>[3x]METLFSGIQPSGIPTIGNYIGALKQFVDVQNDYDCYFCIVDQHAITMPQDRLKLRKQTRQLAAIYLASGIDPDKATLFIQSEVPAHVQAGWMLTTIASVGELERMTQYKDKAQKAVEGIPAGLLTYPPLMAADIVLYNTNIVPVGDDQKQHIELTRNLVDRFNSRYNDVLVKPEIRMPKVGGRVMSLQDPTRKMSKSDDNAKNFISLLDEPNVAAKKIKSAVTDSDGIIKFDRDNKPGITNLISIYAGLTDMPIKDIEAKYEGEGYGKFKGDLAEIVKAFLVEFQEKYESFYNSDKLDDILDQGRDKAHKVSFKTVKKMEKAMGLGRKRHHHHHH

Chuangxinmycin (CXM) is a promising antimicrobial compound targeting bacterial tryptophanyl-tRNA synthetase (TrpRS), an essential enzyme in protein synthesis. TrpRS catalyzes the ligation of Trp to its cognate tRNA, forming tryptophanyl-tRNA (Trp-tRNA), which is required for the accurate translation of genetic codes into proteins. Importantly, bacterial TrpRS exhibits significant structural and functional differences compared to its mammalian counterpart, making it an attractive target for the development of selective antibiotics. Structurally, CXM is a tryptophan (Trp) mimic but is characterized by a unique dihydrothiopyran heterocycle, which distinguishes it from other known antibiotics and contributes to its distinct physicochemical properties.

To ensure rigorous structural comparative analysis, we also determined the structures of SaTrpRS in the absence of substrates or inhibitors (apo-SaTrpRS) and SaTrpRS in complex with Trp (SaTrpRS/Trp complex) at resolutions of 3.04 Å and 2.32 Å, respectively (ESI†). These structures share a similar three-chain asymmetric unit with the SaTrpRS/CXM complex. The CXM complexes show high conformational similarity to Trp complexes and apo proteins (ESI†).> MDYKDDDDKHMSLVLNDLLICCRQLEHDRATERKKEVEKFKRLIRDPETIKHLDRHSDSKQGKYLNWDAVFRFLQKYIQKETECLRIAKPNVSASTQASRQKKMQEISSLVKYFIKCANRRAPRLKCQELLNYIMDTVKDSSNGAIYGADCSNILLKDILSVRKYWCEISQQQWLELFSVYFRLYLKPSQDVHRVLVARIIHAVTKGCCSQTDGLNSKFLDFFSKAIQCARQEKSSSGLNHILAALTIFLKTLAVNFRIRVCELGDEILPTLLYIWTQHRLNDSLKEVIIELFQLQIYIHHPKGAKTQEKGAYESTKWRSILYNLYDLLVNEISHIGSRGKYSSGFRNIAVKENLIELMADICHQVFNEDTRSLEISQSYTTTQRESSDYSVPCKRKKIELGWEVIKDHLQKSQNDFDLVPWLQIATQLISKYPASLPNCELSPLLMILSQLLPQQRHGERTPYVLRCLTEVALCQDKRSNLESSQKSDLLKLWNKIWCITFRGISSEQIQAENFGLLGAIIQGSLVEVDREFWKLFTGSACRPSCPAVCCLTLALTTSIVPGTVKMGIEQNMCEVNRSFSLKESIMKWLLFYQLEGDLENSTEVPPILHSNFPHLVLEKILVSLTMKNCKAAMNFFQSVPECEHHQKDKEELSFSEVEELFLQTTFDKMDFLTIVRECGIEKHQSSIGFSVHQNLKESLDRCLLGLSEQLLNNYSSEITNSETLVRCSRLLVGVLGCYCYMGVIAEEEAYKSELFQKAKSLMQCAGESITLFKNKTNEEFRIGSLRNMMQLCTRCLSNCTKKSPNKIASGFFLRLLTSKLMNDIADICKSLASFIKKPFDRGEVESMEDDTNGNLMEVEDQSSMNLFNDYPDSSVSDANEPGESQSTIGAINPLAEEYLSKQDLLFLDMLKFLCLCVTTAQTNTVSFRAADIRRKLLMLIDSSTLEPTKSLHLHMYLMLLKELPGEEYPLPMEDVLELLKPLSNVCSLYRRDQDVCKTILNHVLHVVKNLGQSNMDSENTRDAQGQFLTVIGAFWHLTKERKYIFSVRMALVNCLKTLLEADPYSKWAILNVMGKDFPVNEVFTQFLADNHHQVRMLAAESINRLFQDTKGDSSRLLKALPLKLQQTAFENAYLKAQEGMREMSHSAENPETLDEIYNRKSVLLTLIAVVLSCSPICEKQALFALCKSVKENGLEPHLVKKVLEKVSETFGYRRLEDFMASHLDYLVLEWLNLQDTEYNLSSFPFILLNYTNIEDFYRSCYKVLIPHLVIRSHFDEVKSIANQIQEDWKSLLTDCFPKILVNILPYFAYEGTRDSGMAQQRETATKVYDMLKSENLLGKQIDHLFISNLPEIVVELLMTLHEPANSSASQSTDLCDFSGDLDPAPNP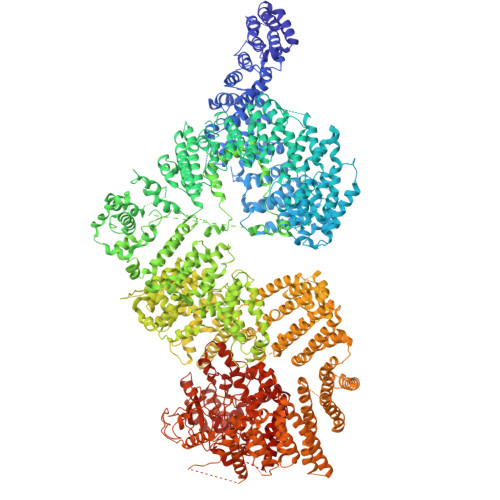PHFPSHVIKATFAYISNCHKTKLKSILEILSKSPDSYQKILLAICEQAAETNNVYKKHRILKIYHLFVSLLLKDIKSGLGGAWAFVLRDVIYTLIHYINQRPSCIMDVSLRSFSLCCDLLSQVCQTAVTYCKDALENHLHVIVGTLIPLVYEQVEVQKQVLDLLKYLVIDNKDNENLYITIKLLDPFPDHVVFKDLRITQQKIKYSRGPFSLLEEINHFLSVSVYDALPLTRLEGLKDLRRQLELHKDQMVDIMRASQDNPQDGIMVKLVVNLLQLSKMAINHTGEKEVLEAVGSCLGEVGPIDFSTIAIQHSKDASYTKALKLFEDKELQWTFIMLTYLNNTLVEDCVKVRSAAVTCLKNILATKTGHSFWEIYKMTTDPMLAYLQPFRTSRKKFLEVPRFDKENPFEGLDDINLWIPLSENHDIWIKTLTCAFLDSGGTKCEILQLLKPMCEVKTDFCQTVLPYLIHDILLQDTNESWRNLLSTHVQGFFTSCLRHFSQTSRSTTPANLDSESEHFFRCCLDKKSQRTMLAVVDYMRRQKRPSSGTIFNDAFWLDLNYLEVAKVAQSCAAHFTALLYAEIYADKKSMDDQEKRSLAFEEGSQSTTISSLSEKSKEETGISLQDLLLEIYRSIGEPDSLYGCGGGKMLQPITRLRTYEHEAMWGKALVTYDLETAIPSSTRQAGIIQALQNLGLCHILSVYLKGLDYENKDWCPELEELHYQAAWRNMQWDHCTSVSKEVEGTSYHESLYNALQSLRDREFSTFYESLKYARVKEVEEMCKRSLESVYSLYPTLSRLQAIGELESIGELFSRSVTHRQLSEVYIKWQKHSQLLKDSDFSFQEPIMALRTVILEILMEKEMDNSQRECIKDILTKHLVELSILARTFKNTQLPERAIFQIKQYNSVSCGVSEWQLEEAQVFWAKKEQSLALSILKQMIKKLDASCAANNPSLKLTYTECLRVCGNWLAETCLENPAVIMQTYLEKAVEVAGNYDGESSDELRNGKMKAFLSLARFSDTQYQRIENYMKSSEFENKQALLKRAKEEVGLLREHKIQTNRYTVKVQRELELDELALRALKEDRKRFLCKAVENYINCLLSGEEHDMWVFRLCSLWLENSGVSEVNGMMKRDGMKIPTYKFLPLMYQLAARMGTKMMGGLGFHEVLNNLISRISMDHPHHTLFIILALANANRDEFLTKPEVARRSRITKNVPKQSSQLDEDRTEAANRIICTIRSRRPQMVRSVEALCDAYIILANLDATQWKTQRKGINIPADQPITKLKNLEDVVVPTMEIKVDHTGEYGNLVTIQSFKAEFRLAGGVNLPKIIDCVGSDGKERRQLVKGRDDLRQDAVMQQVFQMCNTLLQRNTETRKRKLTICTYKVVPLSQRSGVLEWCTGTVPIGEFLVNNEDGAHKRYRPNDFSAFQCQKKMMEVQKKSFEEKYEVFMDVCQNFQPVFRYFCMEKFLDPAIWFEKRLAYTRSVATSSIVGYILGLGDRHVQNILINEQSAELVHIDLGVAFEQGKILPTPETVPFRLTRDIVDGMGITGVEGVFRRCCEKTMEVMRNSQETLLTIVEVLLYDPLFDWTMNPLKALYLQQRPEDETELHPTLNADDQECKRNLSDIDQSFNKVAERVLMRLQEKLKGVEEGTVLSVGGQVNLLIQQAIDPKNLSRLFPGWKAWV> SNAMKNYTLISPCFFGMEKMLAREITNLGYEIIKTEDGRITYKTDEFGIAKSNMWLRCAERVHLKIAEFEAKSFDE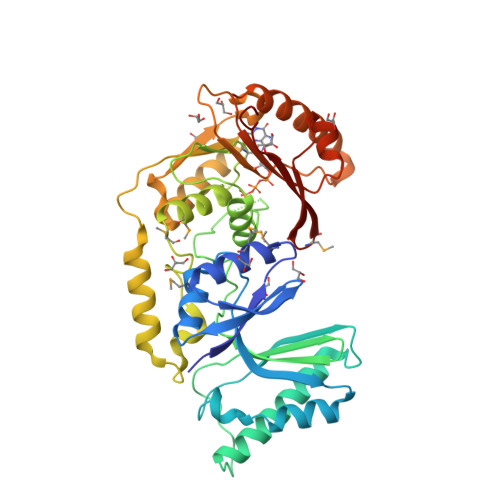LFENTKRINWSRYIPYGAQFPISKASSIKSKLYSTPDVQAIVKKAIVESLKKSYLEDGLLKEDKEKYPIFVFIHKDKVTISIDTTGDALHKRGYREKANKAPIRETLAAGLIYLTPWKAGRVLVDPMCGSGTILIEAAMIGINMAPGLNREFISEKWRTLDKKIWWDVRKDAFNKIDNESKFKIYGYDIDEESIDIARENAEIAGVDEYIEFNVGDATQFKSEDEFGFIITNPPYGERLEDKDSVKQLYKELGYAFRKLKNWSYYLITSYEDFEYEFGQKADKKRKLYNGMLKTNFFQYPGPKPPRNNK>[2x]MIVMRVKVN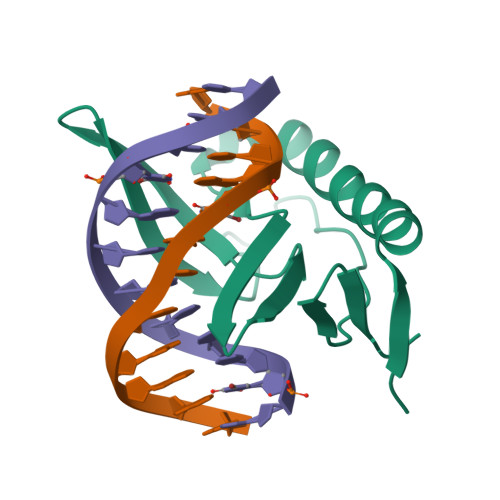EKQFDMIIDKLKLMVYEYNTKIKEYGVYLKPYHIVYKNSKRYIYIGKYWYKLEKIGGKLKWIYLGKTKPIQNMPNPPQIPESTIIKEDNEYIVDEKILYDLE>[2x]GGDSEMAVFGAAAPYLRKSEKERLEAQTRPFDLKKDVFVPDDKQEFVKAKIVSREGGKVTAETEYGKTVTVKEDQVMQQNPPKFDKIEDMAMLTFLHEPAVLYNLKDRYGSWMIYTYSGLFCVTVNPYKWLPVYTPEVVAAYRGKKRSEAPPHIFSISDNAYQYMLTDRENQSILITGESGAGKTVNTKRVIQYFAVIAAIGDRSK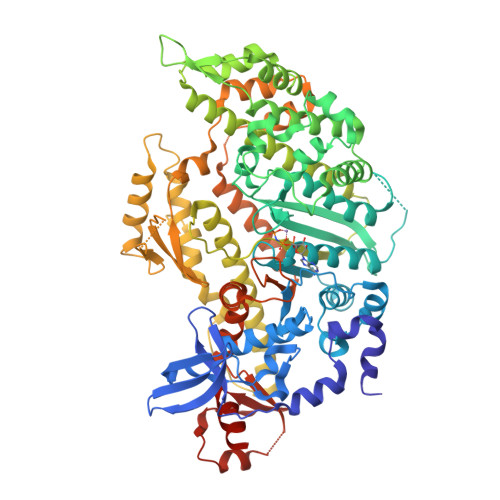KDQSPGKGTLEDQIIQANPALEAFGNAKTVRNDNSSRFGKFIRIHFGATGKLASADIETYLLEKSRVIFQLKAERDYHIFYQILSNKKPELLDMLLITNNPYDYAFISQGETTVASIDDAEELMATDNAFDVLGFTSEEKNSMYKLTGAIMHFGNMKFKLKQREEQAEPDGTEEADKSAYLMGLNSADLLKGLCHPRVKVGNEYVTKGQNVQQVIYATGALAKAVYERMFNWMVTRINATLETKQPRQYFIGVLDIAGFEIFDFNSFEQLCINFTNEKLQQFFNHHMFVLEQEEYKKEGIEWTFIDFGMDLQACIDLIEKPMGIMSILEEECMFPKATDMTFKAKLFDNHLGKSANFQKPRNIKGKPEAHFSLIHYAGIVDYNIIGWLQKNKDPLNETVVGLYQKSSLKLLSTLFANYAGADAPIEKGKGKAKKGSSFQTVSALHRENLNKLMTNLRSTHPHFVRCIIPNETKSPGVMDNPLVMHQLRCNGVLEGIRICRKGFPNRILYGDFRQRYRILNPAAIPEGQFIDSRKGAEKLLSSLDIDHNQYKFGHTKVFFKAGLLGLLEEMRDERLSR>[2x]MLEKTFYKMMLSKSFPFPVEVTYWDGKSEVYGNGTPEIHITFNEKIPMSDITKNASLALGEAYMDKKIEIQGSIQELINGAYQSADSFMRSSKFRKFLPKSKHTEKQSEEDVQSHYDIGNDFYKLWLDPTMTYSCAYFTDDNKDDLEQAQIAKVHHILNKLHPEKGKTLLDIGCGWGTLMLTAAKEYGLKVTGVTLSEEQYKLVQKKI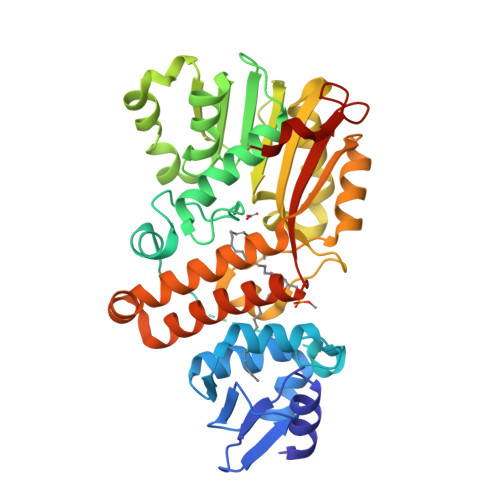YDEGLEDVAEVKLEDYRELGDQQWDYVTSVGMFEHVGSENLGEYFKDVAKYLKNDGVALIHGITRQQGGATNAWINKYIFPGGYIPGLVEIISRIEEANLQVSDVEMLRRHYQRTLEIWDKNFNNARPEIEKNMGERFCRMWDLYLQACAASFESGNIDVVQYLLTKGPSGKSLPMTRKYMLNDKHHHHHH> GGNKLTESRSQSMIVACRKIIRRSIVASNPLELAVEIANKTVIDTEPLKSCLAAIDGGDVA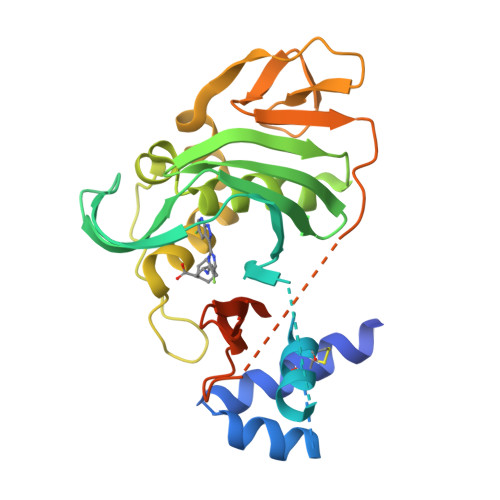CDIIRAALGLKIRQRQRFGRLELKRISGRGFKNDEEILIGNGTIQKIGIWDGEEEFHVRCGECRGILKKSKMKLEKLLINSAKKEDMRDLIILCMVFSQDTRMFQGVRGEINFLNRAGQLLSPMYQLQRYFLNRSNDLFDQWGYEESPKASELHGINESMNASDYTLKGVVVTRNVIDDFSSTETEKVSITKNLSLIKRTGEVIMGANDVSELESQAQLMITYDTPKMWEM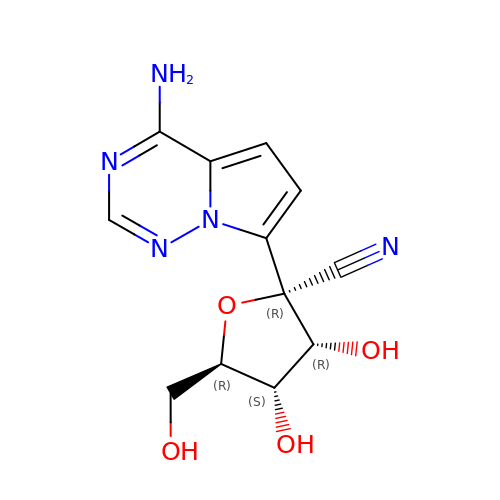(2~{R},3~{R},4~{S},5~{R})-2-(4-azanylpyrrolo[2,1-f][1,2,4]triazin-7-yl)-5-(hydroxymethyl)-3,4-bis(oxidanyl)oxolane-2-carbonitrile | C12 H13 N5 O4 | BRDWIEOJOWJCLU-LTGWCKQJSA-N> MLYID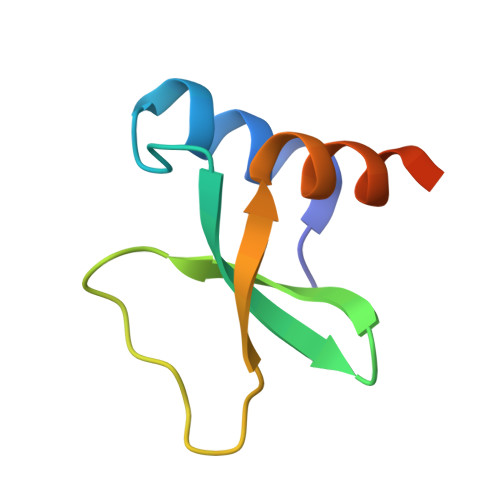EFKEAIDKGYILGDTVAIVRKNGKIFDYVLPHEKVRDDEVVTVERVEEVMVELDKLEHHHHHH>[3x]LPSGSDPAFSQPKSVLDAGLTCQGASPSSVSKPILLVPGTGTTGPQSFDSNWIPLSTQLGYTPCWISPPPFMLNDTQVNTEYMVNAITALYAGSGNNKLPVLTWSQGG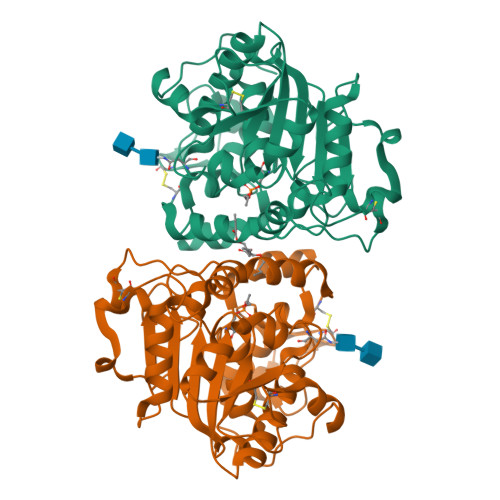LVAQWGLTFFPSIRSKVDRLMAFAPDYKGTVLAGPLDALAVSAPSVWQQTTGSALTTALRNAGGLTQIVPTTNLYSATDEIVQPQVSNSPLDSSYLFNGKNVQAQAVCGPLFVIDHAGSLTSQFSYVVGRSALRSTTGQARSADYGITDCNPLPANDLTPEQKVAAAALLAPAAAAIVAGPKQNCEPDLMPYARPFAVGKRTCSGIVTP>SSGARVEELNKLIQEFTKHDQREYDDQRALEIHTAKDFIFSMLGMVQKLDQKLPVANEYLLLSGGVREGVVDLDLDELNVYARGTDYDMDFTLLVPALKLHDRNQPVTLDMRHSALCHSWLSLRLFDEGTISKWKDCCTIVDHINGATNYFFSPTKVADWFYDSISIVLSEIQKKPQRGMPKVEKVEKNGTIISIILGVGSSRMLYDIVPVVSFKGWPAVAQSWLMENHFWDGKITEEEVISGFYLVPACSYKGKKDNEWRLSFARSEVQLKKCISSSLMQAYQACKAIIIKLLSRPKAISPYHLRSMMLWACDRLPANYLAQEDYAAHFLLGLIDDLQHCLVNKMCPNYFIPQCNMLEHLSEETVMLHARKLSSVRSDPAEHLRTAIEHVKAANRLTLELQRRGSTTSIPSPQSDGGDPN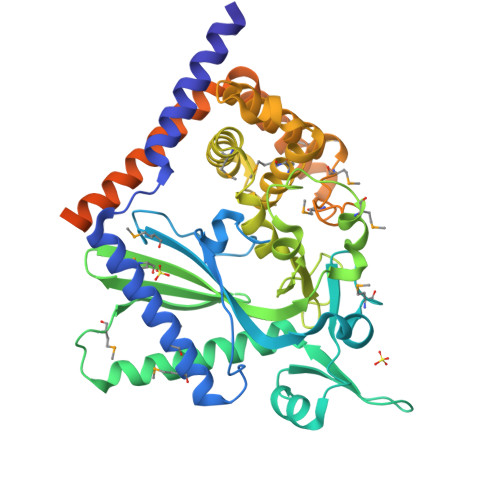QPDDRLAKKLQQLVTENPGKSISVFINPDDVTRPHFRIDDKFF[2x]> AITIGNKNDD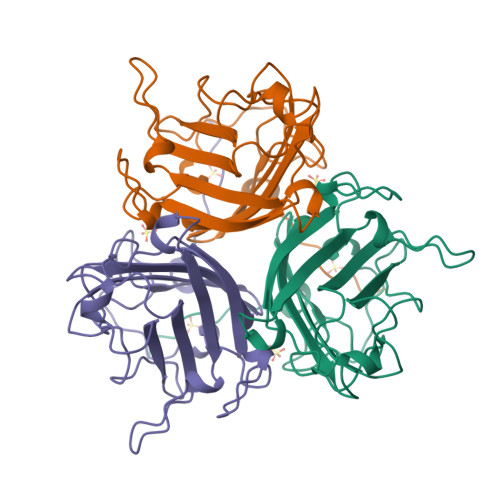KLTLWTTPDPSPNCRIHSDNDCKFTLVLTKCGSQVLATVAALAVSGDLSSMTGTVASVSIFLRFDQNGVLMENSSLKKHYWNFRNGNSTNANPYTNAVGFMPNLLAYPKTQSQTAKNNIVSQVYLHGDKTKPMILTITLNGTSESTETSEVSTYSMSFTWSWESGKYTTETFATNSYTFSYIAQE>MAVPETRPNHTIYINNLNEKIKKDELKKSLHAIFSRFGQILDIL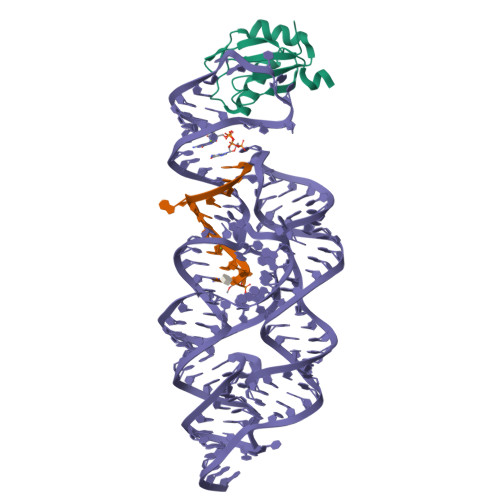VSRSLKMRGQAFVIFKEVSSATNALRSMQGFPFYDKPMRIQYAKTDSDIIAKMK[4x]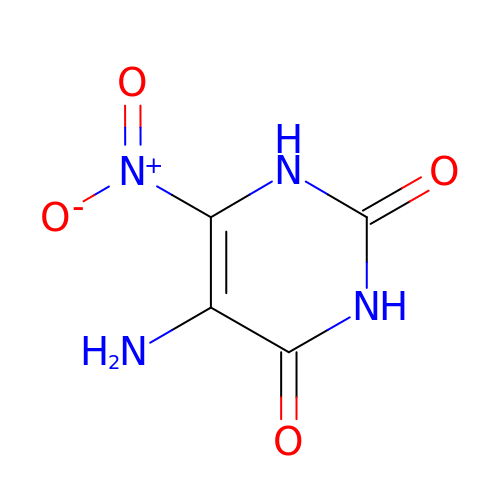5-AMINO-6-NITROPYRIMIDINE-2,4(1H,3H)-DIONE | C4 H4 N4 O4 | CLOSWQFGCBFNCK-UHFFFAOYSA-N>EELPAPVKAIEKQGITIIKTFDAPGGMKGYLGKYQDMGVTIYLTPDGKHAISGYMYNEKGENLSNTLIEKEIYAPAGREMWQRMEQSHWLLDGKKDAPVIVYVFADPFCPYCEQFWQQARPWVDSGKVQLRTLLVGVIKPESPATAAAILASKDPAKTWQQYEASGGKLKLNVPANVSTEQMKVLSDNEKLMDDLGANVTPAIYYMSKENTLQQAVGLPDQK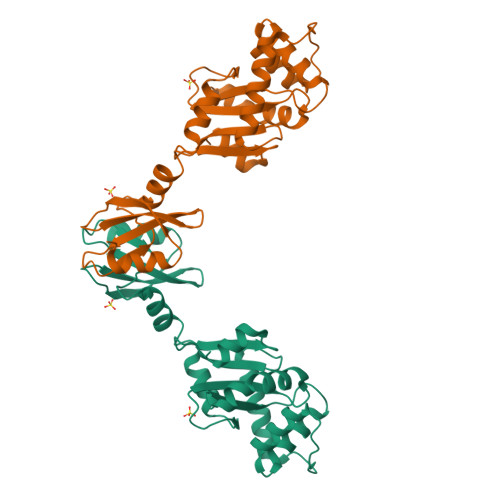TLNIIMGNKHHHHHH[2x]>[2x]MAHHHHHHMNCNYNCVTLHNSVRMPQLGLGVWRAQDGAETANAVRWAIEAGYRHIDTAYIYSNERGVGQGIRESGVPREEVWVTTKVWNSDQGYEKTLAAFERSRELLGLEYIDLYLIHWPGKKKFVDTWKALEKLYEEKKVRAIGVSNFEPHHLTELFKSCKIRPMVNQVELHPLF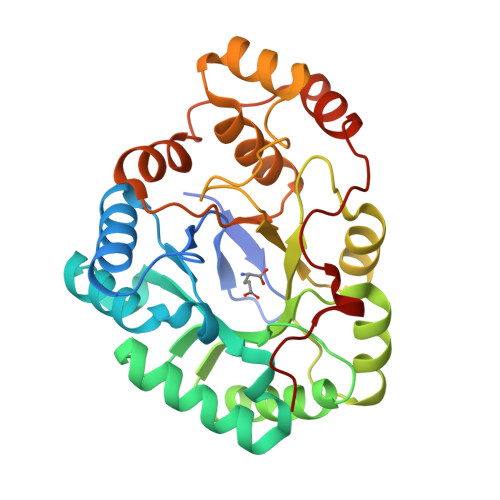QQRTLREFCKQHNIAITAWSPLGSGEEAGILKNHVLGEIAKKHNKSPAQVVIRWDIQHGIVTIPKSTNKGRIQENFNVWDFKLTEEEMRQIDELNEDKRIGADPDNFFPGGEE> ADTIVAVELDSYPNTDIGDPSYPHIGIDIKSIRSKSTARWNMQTGKVGTAHISYNSVAKRLSAVVSYSGTSSTTVSYDVDLNNVLPEWVRVGLSATTGLYKETNTILSWSFTSKLKTNSIADANSLHFSFSQFSQNPKDLILQGDATTDSDGNLQLTRVSSDGSPQGSSVGRALFYAPVHIWEKSAVVASFDATFTFLIKSPDRDPADGITFFIANTDTSIPSGSGGRLLG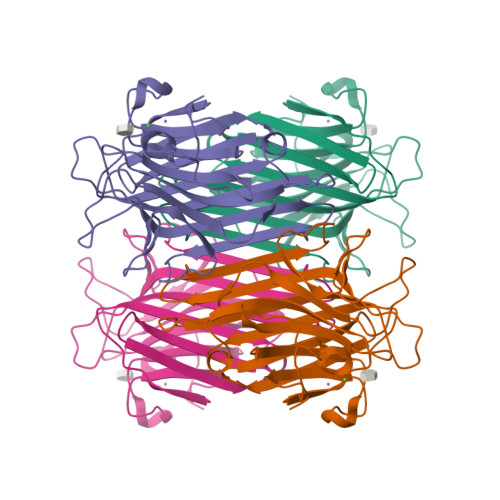LFPDAN> IV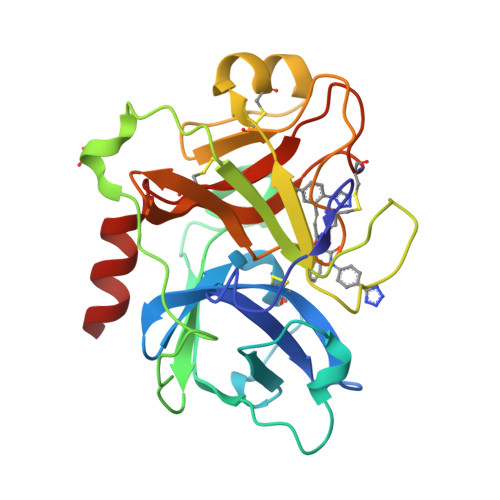GGTASVRGEWPWQVTLHTTSPTQRHLCGGSIIGNQWILTAAHCFYGVESPKILRVYSGILNQAEIAEDTSFFGVQEIIIHDQYKMAESGYDIALLKLETTVNYADSQRPISLPSKGERNVIYTDCWVTGWGYRKLRDKIQNTLQKAKIPLVTNEECQKRYRGHKITHKMICAGYREGGKDACKGDSGGPLSCKHNEVWHLVGITSWGEGCAQRERPGVYTNVVEYVDWILEKTQAV>GSHMTTTEAGASAPSPAVDGAVNQTARQAEADGTDIVTDHDRGVHGYHKQKAEHLKRLRRIEGQIRGLQRMVDEDVYCIDILTQ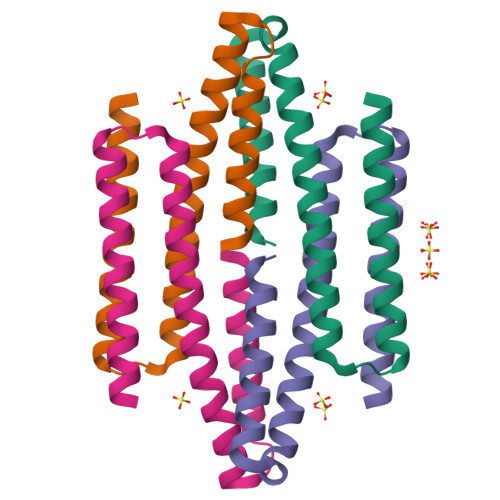VSASTKALQSFALQLLEEHLRHCVADAALKGGTEIDAKVEEATKAIGRLLRT[2x]>[2x]MASWSHPQFEKGADDDDKVPDPTSVDSVKYSKIKGIPKLDDANDAGGKHSLECTLILTEGDSAKSLAVSGLGVIGRDRYGVFPLRGKILNVREASHKQIMENAEINNIIKIVGLQYKKSYDDAESLKTLRYGKIMIMTDQDQDGSHIKGLLINFIHHNWPSLLKHGFLEEFITPIVKASKNKQELSFYSIPEFDEWKKHIENQKAWKIKYYKGLGTSTAKEAKEYFADMERHRILFRYAGPEDDAAITLAFSKKKIDDRKEWLTNFMEDRRQRRLHGLPEQFLYGTATKHLTYNDFINKELILFSNSDNERSIPS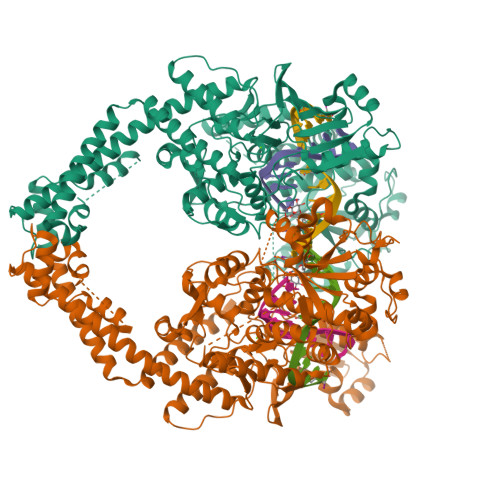LVDGFKPGQRKVLFTCFKRNDKREVKVAQLAGSVAEMSAYHHGEQALMMTIVNLAQNFVGSNNINLLQPIGQFGTRLHGGKDAASPRYIFTMLSTLARLLFPAVDDNLLKFLYDDNQRVEPEWYIPIIPMVLINGAEGIGTGWACKLPNYDAREIVNNVRRMLDGLDPHPMLPNYKNFKGTIQELGQNQYAVSGEIFVVDRNTVEITELPVRTWTQVYKEQVLEPMLNGTDKTPALISDYKEYHTDTTVKFVVKMTEEKLAQAEAAGLHKVFKLQTTLTCNSMVLFDHMGCLKKYETVQDILKEFFDLRLSYYGLRKEWLVGMLGAESTKLNNQARFILEKIQGKITIENRSKKDLIQMLVQRGYESDPVKAWKEAQEKAAEEDETQNQHDDSSSDSGTPSGPDFNYILNMSLWSLTKEKVEELIKQRDAKGREVNDLKRKSPSDLWKEDLAAFVEELDKVESQEREDGAPGFSSISAHHHHHHHHHH>[4x]SNAMEPVSSWGNTSLVSVDPEIHDLIEKEKRRQCRGIELIASENFTSFAVIEALGSALTNKYSEGIPGNRYYGGNEFIDEIENLCRSRALEAFHCDPAAWGVNVQPYSGSPANFAAYTALLQPHDRIMGLDLPSGGHLTHGYYTSGGKKISATSIYFESLPYKVNFTTGYIDYDKLEEKALDFRPKLLIC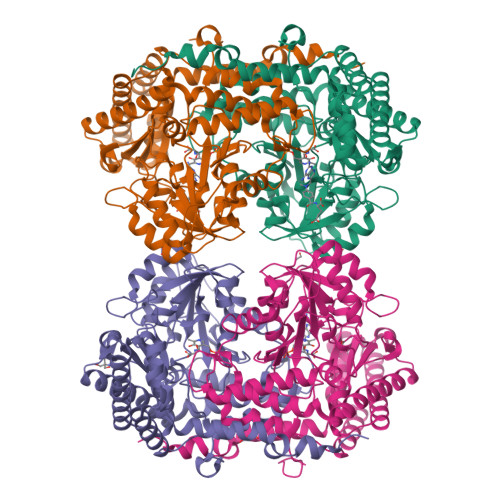GGSAYPRDWDYARFRAIADKVGALLLCDMAHISGLVAAQEAANPFEYCDVVTTTTHKSLRGPRAGMIFYRKGPKPPKKGQPEGAVYDFEDKINFAVFPALQGGPHNHQIGALAVALKQANTPGFKVYAKQVKANAVALGNYLMSKGYQIVTNGTENHLVLWDLRPLGLTGNKVEKLCDLCSITLNKNAVFGDSSALAPGGVRIGAPAMTSRGLVEKDFEQIGEFLSRAVTLTLDIQKTYGKLLKDFNKGLVNNKDLDQLKADVEKFSASYEMPGFLMSEMKYKD> GHMQETQAVEAGEKTVEQFVQALNKGDYNKAAEMTSKKAANKSALSEKEILDKYQNIYGAADVKGLQISNLKVDKKDDSTYSFSYKAKMNTSLGELKDLSYKGTLDRNDGQ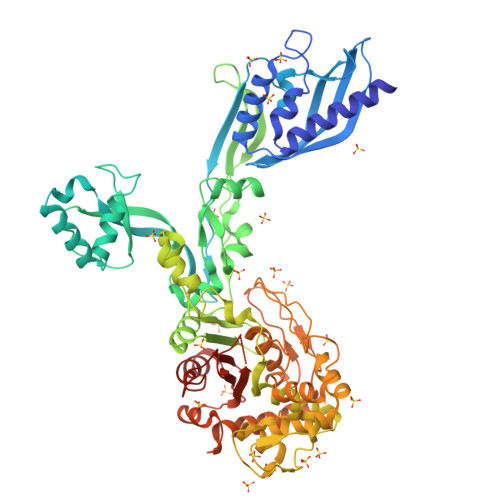TTINWQPNLVFPEMEGNDKVSLTTQEAARGNIIDRNGEPLATTGKLKQLGVVPSKLGDGGEKTANIKAIASSFDLTEDAINQAISQSWVQPDYFVPLKIIDGATPELPAGATIQEVDGRYYPLGEAAAQLIGYVGDITAEDIDKNPELSSNGKIGRSGLEMAFDKDLRGTTGGKLSITDADGVEKKVLIEHEVQNGKDIKLTIDAKAQKTAFDSLGGKAGSTVATTPKTGDLLALASSPSYDPNKMTNGISQEDYKAYEENPEQPFISRFATGYAPGSTFKMITAAIGLDNGTIDPNEVLTINGLKWQKDSSWGSYQVTRVSDVSQVDLKTALIYSDNIYTAQETLKMGEKKFRTGLDKFIFGEDLDLPISMNPAQISNEDSFNSDILLADTGYGQGELLINPIQQAAMYSVFANNGTLVYPKLIADKETKDKKNVIGETAVQTIVPDLREVVQDVNGTAHSLSALGIPLAAKTGTAEIGGGGGGGGKENSFLFAFNPDNQGYMMVSMLENKEDDDSATKRASELLQYLNQNYQ> N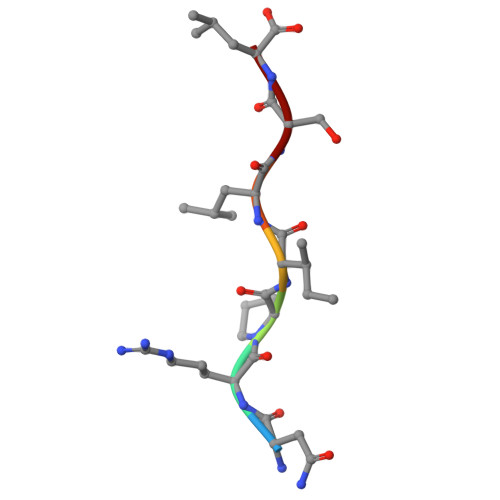RPILSL>TRRTAFFFDELCLWHAAGPHALTLPVGGWVQPPAAAGHAESPETKRRLKSLLDVSGLTARLQLRSAPPASDEDLLRVHPAHYLERFKALSDAGGGSLGQDAPIGPGSYEIARLSAGLAIAALDAVLAGEADNAYSLSRPPGAHCLPDQAMGFCFFANIAVAIEAAKARHGVERVAVLDWDVHHGNGTQAIYYRRDDVLSISLHQDGCFPPGYSGAEDIGEDRGRGFNLNVPLLPGGGHDAYMQAMQRIVLPALERFRPQLIVVASGFDANAVDPLARMQLHSDSFRAMTAMVRDAAERHAG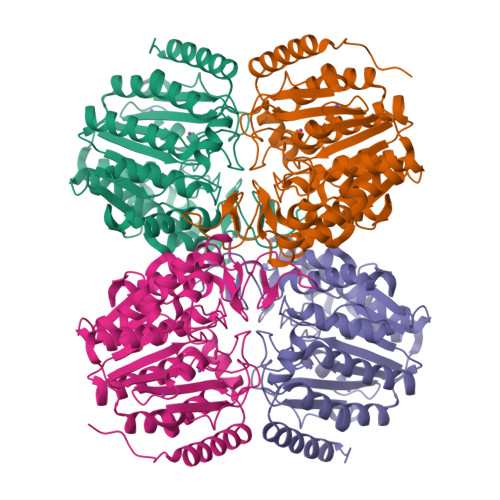GRLVVVHEGGYSEAYVPFCGLAVIEELSGVRSAVRDPLRDFIELQQPNAAFRDFQRQRLEELAAQFGLCPAQPLQAAR[2x]> MKIVYWSGTGNTEKMAELIAKGIIESGKDVNTINVSDVNIDELLNEDILILGCSAMGPEVLEESEFEPFIEEISTKISGKKVALFGSYG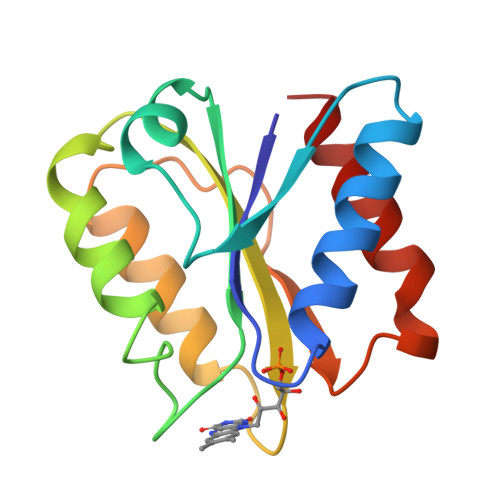WGDGKWMRDFEERMNGYGCVVVETPLIVQNEPDEAEQDCIEFGKKIANI1-[2-[5-[4-(4-azanylbutyl)-3-methyl-1,2,3-triazol-3-ium-1-yl]-2-[4-(2-phenylethyl)-1,3-thiazol-2-yl]phenoxy]ethyl]imidazolidin-2-one | C29 H36 N7 O2 S | 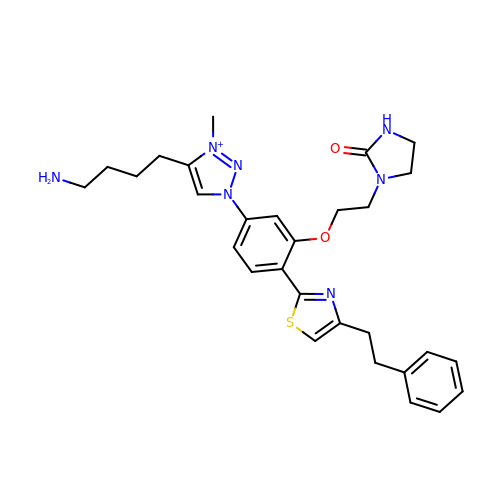OPGOAZPEMDHEOI-UHFFFAOYSA-O Malate dehydrogenase (MDH, EC 1.1.1.37) catalyzes a dehydrogenation reaction from malic acid to generate oxaloacetic acid, which is accompanied by reduced NAD generating NADH. MDH from T. thermophilus (TtMDH) is more similar in amino acid sequence to NADP-dependent chloroplastic MDH than NAD-dependent bacterial and mitochondrial MDHs. The molecular mass of TtMDH in solution determined by analytical gel filtration chromatography was about 61 kDa, so TtMDH is a homodimeric enzyme like most MDHs. Similar to other MDHs, a protomer of TtMDH has the N-terminal NAD binding domain and C-terminal catalytic domain and consists of 12 helices and 11 β-strands.

The crystallographic asymmetric unit contains two subunits, which forms a homodimer arranged through a noncrystallographic two-fold axis and is consistent with the observation of analytical gel filtration chromatography. The two subunits are virtually superimposable, with a root mean square deviation (RMSD) of 0.124 Å between the corresponding Cα atoms of the two subunits. Two monomers are further assembled into a dimer via reciprocal interactions from helices α1, α2, α7, α8, α9, α10, and α11. The dimeric interface is about 1619 Å2 and involves 18 hydrogen bonds and extensive hydrophobic interaction, as analyzed by PDBsum. The overall B-factor of the crystal structure color coded as defined in Figure 4C is quite low, which indicates the high stability of TtMDH. Conversely, the loop region between β4 and α4 reveals higher B-factor values, considered to be involved in conformational changes with NAD binding. However, electron densities in the apo-form crystals were of high quality and generally continuous, so the residues of the entire sequence could be modeled into the structure. Even the electron densities of the loop regions for NAD binding are clearly shown. Crystal structures of apo and NAD-bound forms of TtMDH revealed slight movement of the binding loop and a few structural elements around the binding packet in the presence of NAD. In the cMDH–NAD complex, the mobile loop closed to bring key residues into contact with the co-substrate, but the crystal structure of TtMDH presents an open conformation of the binding loop.

>[2x]MKAPVRVAVTGAAGQIGYSLLFRIAAGEMLGKDQPVILQLLEIPQAMKALEGVVMELEDCAFPLLAGLEATDDPKVAFKDADYALLVGAAPRKAGMERRDLLQVNGKIFTEQGRALAEVAKKDVKVLVVGNPANTNALIAYKNAPGLNPRNFTAMTRLDHNRAKAQLAKKTGTGVDRIRRMTVWGNHSSTMFPDLFHAEVDGRPALELVDMEWYEKVFIPTVAQRGAAIIQARGASSAASAANAAIEHIRDWALGTPEGDWVSMAVPSQGEYGIPEGIVYSFPVTAKDGAYRVVEGLEINEFARKRMEITAQELLDEMEQVKALGLIRKLAAALEHHHHHH> VDEQPLENYLDMEYFGTIGIGTPAQDFTVVFDTGS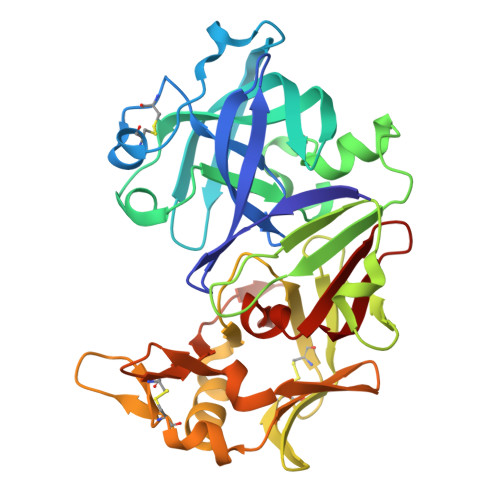SNLWVPSVYCSSLACTNHNRFNPEDSSTYQSTSETVSITYGTGSMTGILGYDTVQVGGISDTNQIFGLSETEPGSFLYYAPFDGILGLAYPSISSSGATPVFDNIWNQGLVSQDLFSVYLSADDQSGSVVIFGGIDSSYYTGSLNWVPVTVEGYWQITVDSITMNGEAIACAEGCQAIVDTGTSLLTGPTSPIANIQSDIGASENSDGDMVVSCSAISSLPDIVFTINGVQYPVPPSAYILQSEGSCISGFQGMNLPTESGELWILGDVFIRQYFTVFDRANNQVGLAPVA> MDIPKITTFLMFNNQAEEAVKLYTSLFEDSEIITMAKYGENGPGDPGTVQHSIFTLNGQVFMAIDANSGTELPISLFVTVKDTIEMERLFNGLKDEGAILMPKTNMPPYREFAWVQD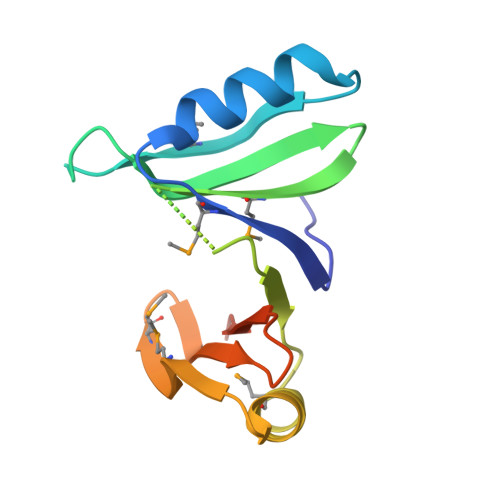KFGVSFQLALPEEGGSHHHHHH> MILQALHGYYQRMSADPDAGMPPYGTSMENISFALVLDAKGTLRGIEDLREQEGKKLRPRKMLVPIAEKKGNGIKPNFLWENTSYILGVDAKGKQERTDKCHAAFIAHIKAYCDTADQDLAAVLQFLEHGEKDLSAFPVSEEVIGSNIVFRIEGEPGFVHERPAARQAWANCLNRREQGLCGQCLITGERQKPIAQLHPSIKGGRDGVRGAQAVASIVSFNNTAFESYGKEQSINAPVSQEAAFSYVTALNYLLNPSNRQKVTIADATVVFWAERSSPAEDIFAGMFDPPSTTAKPESSNGTPPEDSEEGSQPDTARDDPHAAARMHDLLVAIRSGKRATDIMPDMDESVRFHVLGLSPNAARLSVRFWEVDTVGHMLDKVGRHYRELEIIPQFNNEQEFPSLSTLLRQTAVLNKTENISPVLAGGLFRAMLTGGPYPQSLLPAVLGRIRAEHARPEDKSRYRLEVVTYYRAALIKAYLIRNRKLEVPVSLDPARTDRPYLLGRLFAVLEKAQEDAVPGANATIKDRYLASASANPGQVFHMLLKNASNHTAKLRKDPERKGSAIHYEIMMQEIIDNISDFPV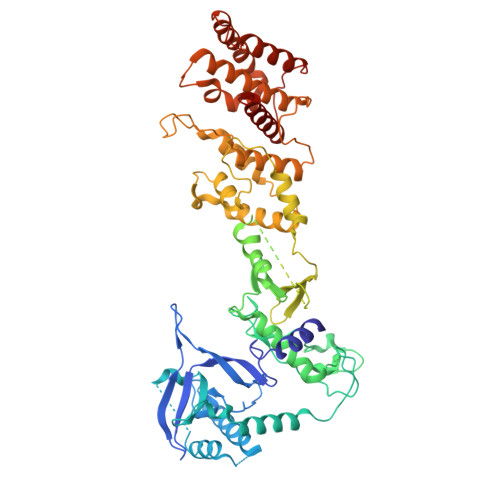TMSSDEQGLFMIGYYHQRKALFTKKNKEN The genome of orthomyxoviruses consists of multiple segments of negative-sense, single-stranded RNA molecules, each packaged in the form of rod-shaped, double-helical ribonucleoprotein (RNP) complexes. Our study of a fish orthomyxovirus, the infectious salmon anemia virus (ISAV), shows that its nucleoprotein (NP), which forms the protein scaffold backbone of the viral RNP, has a bi-lobular structure like the influenza virus NP. Each RNP contains a viral RNA, a heterotrimeric viral polymerase (consisting of PA, PB1, and PB2) and multiple copies of the viral-encoded nucleoprotein (NP) that bind viral RNA in a stoichiometric manner. Our results indicate that each ISAV-NP binds ∼12-nt RNA, shorter than the 24–28 nts originally estimated for the influenza A virus based on population average.

Without the last 16 residues, the ISAV-NP ΔC16 mutant also formed dimers, similar to the full-length protein, and produced crystals that diffracted far better up to 2.7 Å resolution. The crystal structure of the ISAV-NP ΔC16 was determined by single-wavelength anomalous dispersion (SAD). The final model contains 495 amino acid residues in total, including residues 5–25, 27–38, 41–45, 61–75, 86–112, 133–182, 201–320, 325–497, 504–530, and 542–586. Each NP molecule can be divided into three domains: an N-terminal domain, a head domain, and a body domain. While the N-terminal domain is made up of a single polypeptide stretch containing the first 111 residues, the head and body domains are not colinear, with the head domain made from two excursions of the polypeptide chain (residues 272–380 and 494–558) out of the body domain. Structural comparison shows that the head and body domains of ISAV-NP closely resemble those of the influenza A virus NP, despite the lack of significant sequence similarity. Although there is only one NP in each crystallographic asymmetric unit, dimers are found around the crystallographic two-fold symmetry axes, which are presumably the same as those found in the solution. The tail loop of ISAV-NP (residues 504–530) folds into an extended β-hairpin that protrudes into a deep pocket in a neighboring subunit to mediate dimer formation. The ISAV-NP dimer interface is ∼3520 Å2 in size, of which a 1518 Å2 area is mediated by the tail loop alone. Analogous to the influenza A virus NP, there is a potential RNA-binding groove between the head and body domains of the ISAV-NP.

> MGHHHHHHADKGMTYSFDVRDNTLVVRRSTATKSGIKISYREDRGTSLLQKAFAGTEDEFWVELDQDVYVDKKIRKFLEEEKMKDMSTRVSGAVAAAIERSVEFDNFSKEAAANIEMAGVDDEEAGGSGLVDNKRKNKGVSNMAYNLSLFIGMVFPALTTFFSAILSEGEMSIWQNGQAIMRILALADEDGKRQTRTGGQRVDMADVTKLNVVTANGKVKQVEVNLNDLKAAFRQSRPKRSDYRKGQGSKATESSISNQCMALIMKSVLSADQLFAPGVKMMRTNGFNASYTTLAEGANIPSKYLRHMRNCGGVALDLMGMKRIKNSPEGAKSKIFSIIQKKVRGRCRTEEQRLLTSALKISDGENKFQRIMDTLCTSFLIDPPRTTKCFIPPISSLMMYIQEGNSVLAMDFMKNGEDACKICREAKLKVGVNSTFTMSVARTCVAVSMVATAFCSADIIENAVPGSERYRSNIKANTTKPKKDSTYTIQGLRLSNVRYEARPETSQSNTDRSWQVNVTDSFGGLAVFNQGAIREMLGDGTSETTSVNVRALVKRILKSASERSARAVKTFMVGEQGKSAIVISGVGLFSIDFEGVEEAERITDMTP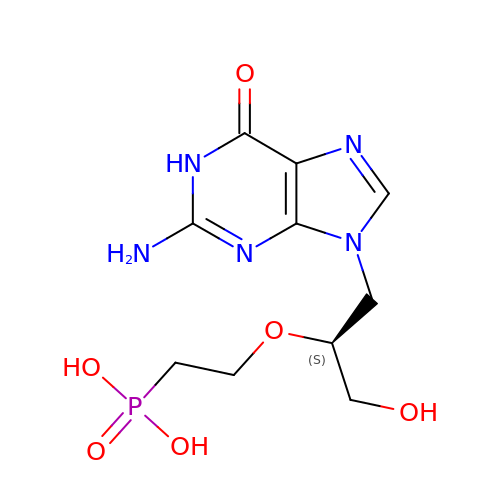(2-{[(2S)-1-(2-amino-6-oxo-1,6-dihydro-9H-purin-9-yl)-3-hydroxypropan-2-yl]oxy}ethyl)phosphonic acid | C10 H16 N5 O6 P | CRTHRZMQPBKEQP-LURJTMIESA-N>WSHPQFEKTPATQPLINAEPAVAAQTEQNPQVGQVMPGVQGADAPVVAQNGPSRDVKLTFAQIAPPPGSMVLRGINPNGSIEFGMRSDEVVTKAMLNLEYTPSPSLLPVQSQLKVYLNDELMGVLPVTKEQLGKKTLAQMPINPLFISDFNRVRLEFVGHYQDVCEKPASTTLWLDVGRSSGLDLTYQTLNVKNDLSHFPVPFFDPSDNRTNTLPMVFAGAPDVGLQQASAIVASWFGSRSGWRGQNFPVLYNQLPDRNAIVFATNDKRPDFLRDHPAVKAPVIEMINHPQNPYVKLLVVFGRDDKDLLQAAKGIAQGNILFRGESVVVNEVKPLLPRKPYDAPNWVRTDRPVTFGELKTYEEQLQSSGLEPAAINVSLNLPPDLYLMRSTGIDMDINYRYTMPPVKDSSRMDISLNNQFLQSFNLSSKQEANRLLLRIPVLQGLLDGKTDVSIPALKLGATNQLRFDFEYMNPMPGGSVDNCITFQPVQNHVVIGDDSTIDFSKYYHFIPMPDLRAFANAGFPFSRMADLSQTITVMPKAPNEAQMETLLNTVGFIGAQTGFPAINLTVTDDGSTIQGKDADIMIIGGIPDKLKDDKQIDLLVQATESWVKTPMRQTPFPGIVPDESDRAAETRSTLTSSGAMAAVIGFQSPYNDQRSVIALLADSPRGYEMLNDAVNDSGKRATMFGSVAVIRESGINSLRVGDVYYVGHLP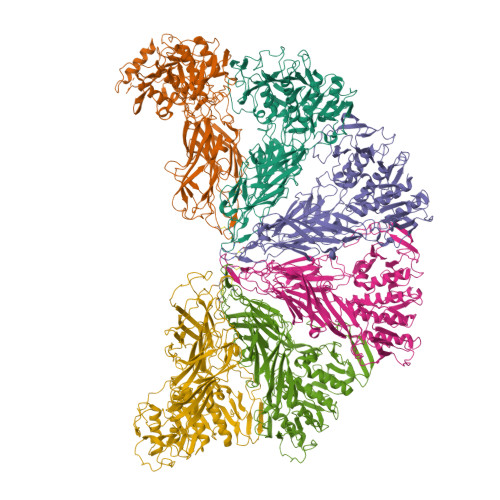WFERVWYALANHPILLAVLAAISVILLAWVLWRLLRIISRRRLNPDNE[6x]> MDYDFKVKLSSERERVEDLFEYEGCKVGRGTYGHVYKAKRKDGKDDKDYALKQIEGTGISMSACREIALLRELKHPNVISLQ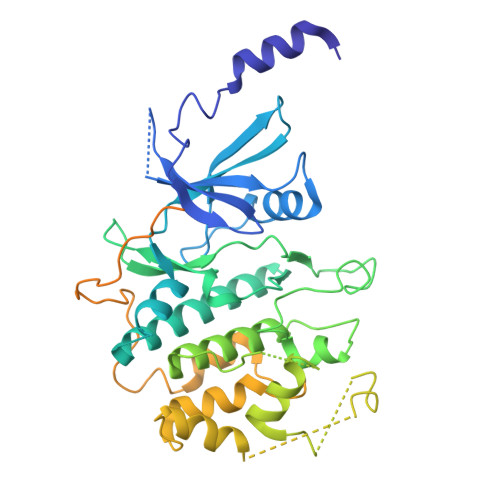KVFLSHADRKVWLLFDYAEHDLWHIIKFHRASKANKKPVQLPRGMVKSLLYQILDGIHYLHANWVLHRDLKPANILVMGEGPERGRVKIADMGFARLFNSPLKPLADLDPVVVTFWYRAPELLLGARHYTKAIDIWAIGCIFAELLTSEPIFHCRQEDIKTSNPYHHDQLDRIFNVMGFPADKDWEDIKKMPEHSTLMKDFRRNTYTNCSLIKYMEKHKVKPDSKAFHLLQKLLTMDPIKRITSEQAMQDPYFLEDPLPTSDVFAGCQIPYPKREFLTEEEPDDKGDKKNQQQQQGNNHTNGTGHPGNQDSSHTQGPPLKKVRVVPPTTTSGGLIMTSDYQRSNPHAAYPNPGPSTSQPQSSMGYSATSQQPPQYSHQTHRY> GPHMKHPLMNVWTLWYLENDRSKSWEDMQNEITSFDTVEDFWSLYNHIKPPSEIKLGSDYSLFKKNIRPMWEDAANKQGGRWVITLNKSSKTDLDNLWLDVLLCLIGEAFDHSDQICGAVINI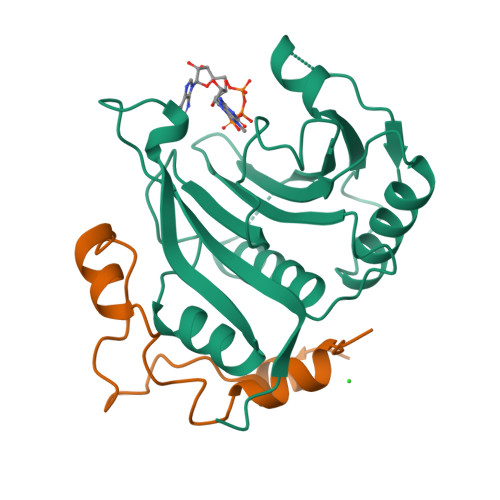RGKSNKISIWTADGNNEEAALEIGHKLRDALRLGRNNSLQYQLHKDTMVKQGSNVKSIYTL;> GPHMLESRVSYDIEHLLYYSMSPHSWTLPTDWQKMQETAPSILRNKDLQDESQRFDGDKYLASIKTAAKR>AMECRLLPYALHKWSSFSSTYLPENILVDKPNDQSSRWSSESNYPPQYLILKLERPAIVQNITFGKYEKTHVCNLKKFKVFGGMNEENMTELLSSGLKNDYNKETFTLKHKIDEQMFPCRFIKIVPLLSWGPSFNFSIWYVELSGIDDPDIVQPC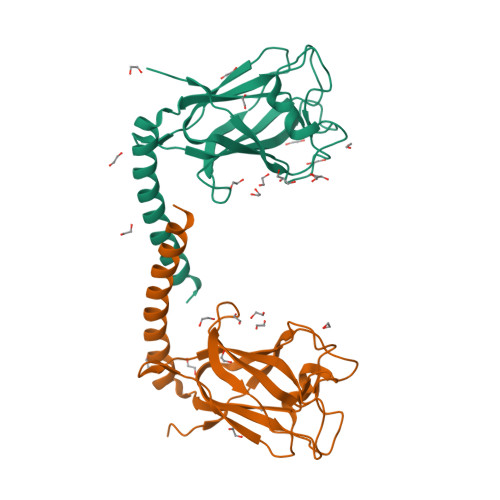LNWYSKYREQEAIRLCLKHFRQHNYTEAFESLQKKTKIALE[2x]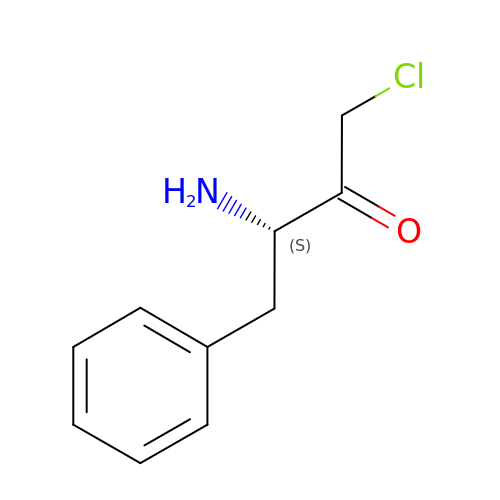PHENYLALANYLMETHYLCHLORIDE | C10 H12 Cl N O | CNNSBPMDYXZFTQ-VIFPVBQESA-N> DEYEIIETIGNGAYGVVSSARRRLTGQQVAIKKIPNAFDVVTNAKRTLRELKILKHFKHDNIIAIKDILRPTVPYGEFKSVYVVLDLMESDLHQIIHSSQPLTLEHVRYFLYQLLRGLKYMHSAQVIHRDLKPSNLLVNENCELKIGDFGMARGLCTSPAEHQYFMTEYV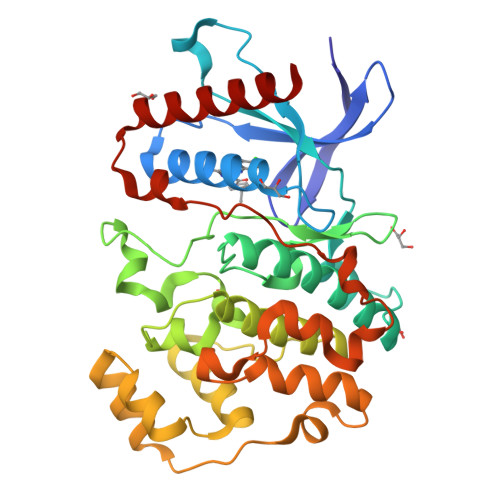ATRWYRAPELMLSLHEYTQAIDLWSVGCIFGEMLARRQLFPGKNYVHQLQLIMMVLGTPSPAVIQAVGAERVRAYIQSLPPRQPVPWETVYPGADRQALSLLGRMLRFEPSARISAAAALRHPFLAKYHDPDDEPDCAPPFDFAFDREALTRERIKEAIVAEIEDFHARRE>AHMAMIKMSPEEIRAKSQSYGQGSDQIRQILSDLTRAQGEIAANWEGQAFSRFEEQFQQLSPKVEK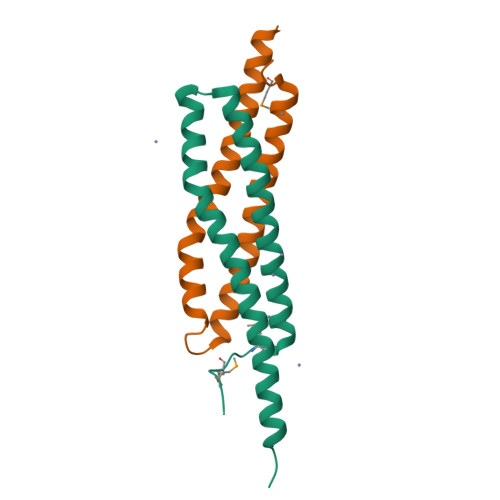FAQLLEEIKQQLNSTADAVQEQDQQLSNNFGLQ[2x]>[2x]SNAEELQALVDNIPAAIYHLDVSGQATIRFRP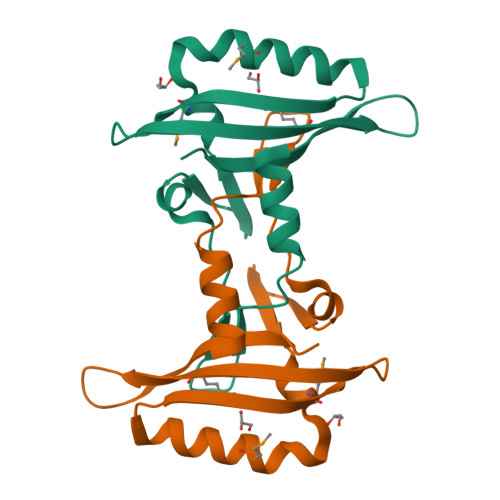PAFLKTLVSEHAGTTRLNTLSMIHHDDRHMLSNAYSKLREAKHSLTLVYRIVTPEGKLHWIEDHMRSSFSDDGLFSGIDGILCEVT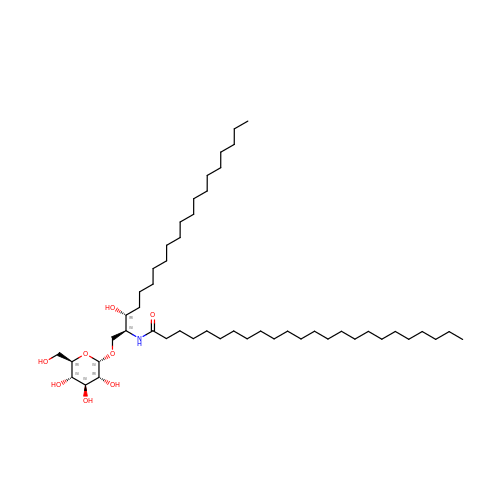N-{1-[(HEXOPYRANOSYLOXY)METHYL]-2-HYDROXYNONADECYL}TETRACOSANAMIDE | C50 H99 N O8 | OOIZAFBOLVYGJT-HDTBOXPDSA-N>TLQIQFKKYELPPLPYKIDALEPYISKDIIDVHYNGHHKGYVNGANSLLERLEKVVKGDLQTGQYDIQGIIRGLTFNINGHKLHALYWENMAPSGKGGGKPGGALADLINKQYGSFDRFKQVFTETANSLPGTGWAVLYYDTESGNLQIMTFENHFQNHIAEIPIILILDEFEHAYYLQYKNKRADYVNAWWNVVNWDAAEKKLQKYL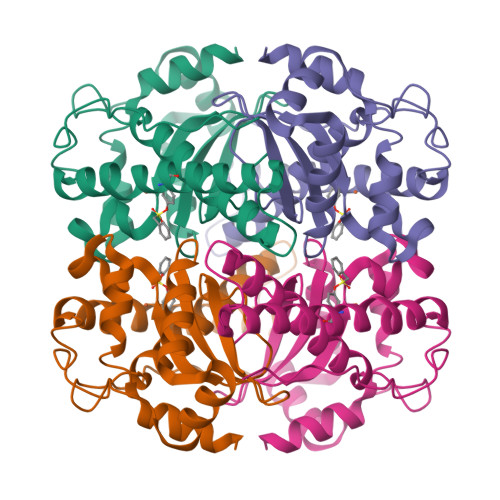TK[2x]> MVREPATEAEAALCAVYAEVLGLDKVGADADFFALGG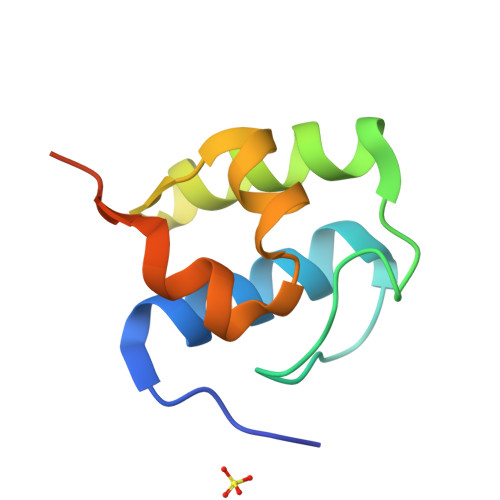DSVLTLRLVHRARSAGWEISARHVFRHPVVADLAAVAQPVTEGSHHHHHH4-(TRIFLUOROMETHYL)BENZENE-1,2-DIAMINE | C7 H7 F3 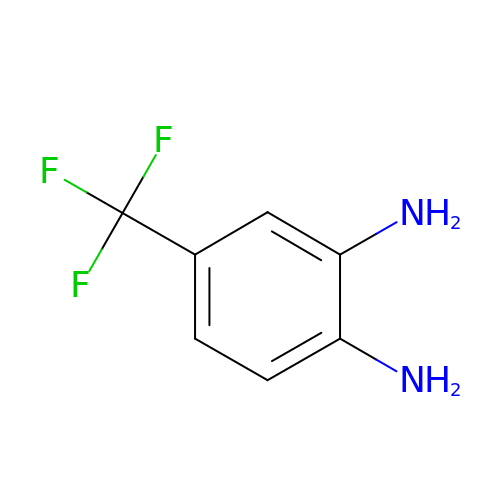N2 | RQWJHUJJBYMJMN-UHFFFAOYSA-N> MAAPILFWHRRDLRLSDNIGLAAARAQSAQLIGLFCLDPQILQSADMAPARVAYLQGCLQELQQRYQQAGSRLLLLQGDPQHLIPQLAQQLQAEAVYWNQDIEPYGRDRDGQVAAALKTAGIRAVQLWDQLLHSPDQILSGSGNPYSVYGPFWKNWQAQPKPTPVATPTELVD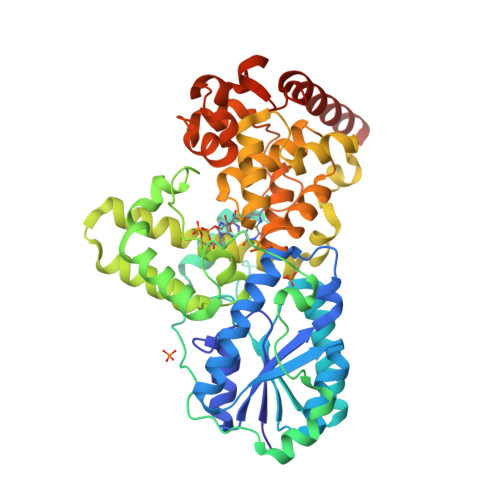LSPEQLTAIAPLLLSELPTLKQLGFDWDGGFPVEPGETAAIARLQEFCDRAIADYDPQRNFPAEAGTSGLSPALKFGAIGIRQAWQAASAAHALSRSDEARNSIRVWQQELAWREFYQHALYHFPSLADGPYRSLWQQFPWENREALFTAWTQAQTGYPIVDAAMRQLTETGWMHNRCRMIVASFLTKDLIIDWRRGEQFFMQHLVDGDLAANNGGWQWSASSGMDPKPLRIFNPASQAKKFDATATYIKRWLPELRHVHPKDLISGEITPIERRGYPAPIVNHNLRQKQFKALYNQLKAAIAEPEAEPDS>[7x]MSSNYVLHTNDGRTIVAEG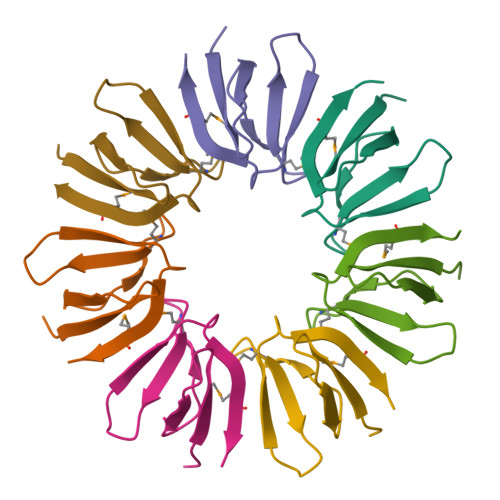KPKVDDETGMISYTDAYGQQQQINRDNVKEMAKGKLEHHHHHH> MLSPEALTTAVDAAQQAIALADTLDVLARVKTEHLGDRSPLALARQALAVLPKEQRAEAGKRVNAARNAAQRSYDERLATLRAERDAAVLVAEGIDVTLPSTRVPAGARHPIIMLAEHVADTFIAMGWELAEGPEVETEQFNFDALNFPADHPARGEQDTFYIAPEDSRQLLRTHTSPVQIRTLLARELPVYIISIGRTFRTDELDATHTPIFHQVEGLAVDRGLSMAHLRGTLDAFARAEFGPSARTRIRPHFFPFTEPSAEVDVWFANKIGGAAWVEWGGCGMVHPNVLRATGIDPDLYSGFAFGMGLERT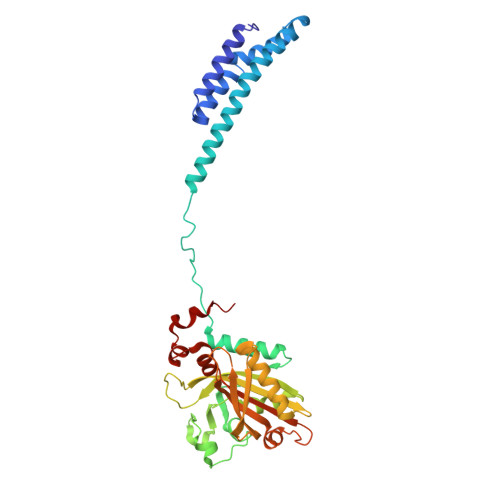LQFRNGIPDMRDMVEGDVRFSLPFGVGA>[2x]SNADEVQVAVAANFTAPIQAIAKEFEKDTGHRLVAAYGATGQFYTQIKNGAPFQVFLSADDSTPAKLEQEGEVVP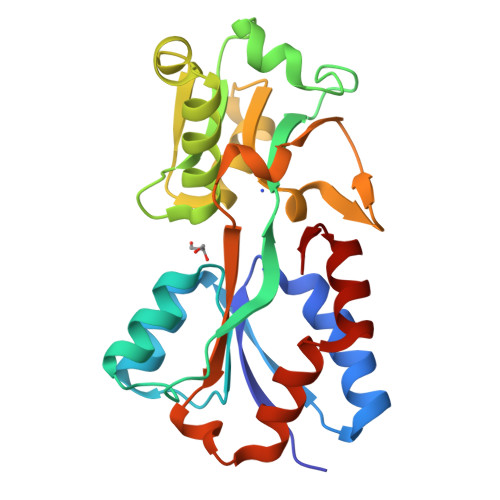GSRFTYAIGTLALWSPKAGYVDAEGEVLKSGSFRHLSIANPKTAPYGLAATQAMDKLGLAATLGPKLVEGQNISQAYQFVSSGNAELGFVALSQIYKDGKVATGSAWIVPTELHDPIRQDAVILNKGKDNAAAKALVDYLKGAKAAALIKSYGYEL> GPLGSPYTIELIQPEDGEAVIAMLKTFFFKDEPLNTFLDLGECKELEKYSLKPLPDNCSYKAVNKKGEIIGVFLNGLMRRPSPDDVPEKAADSCEHPKFKKILSLMDHVEEQFNIFDVYPDEELILDGKILSVDTNYRGLGI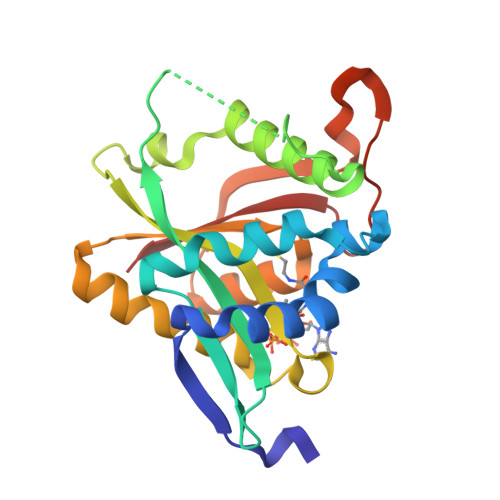AGRLTERAYEYMRENGINVYHVLCSSHYSARVMEKLGFHEVFRMQFADYKPQGEVVFKPAAPHVGIQVMAKEV7-[3-methyl-5-[2-methyl-5-[(pyridin-3-ylamino)methyl]phenyl]imidazol-4-yl]-4~{H}-1,4-benzoxazin-3-one 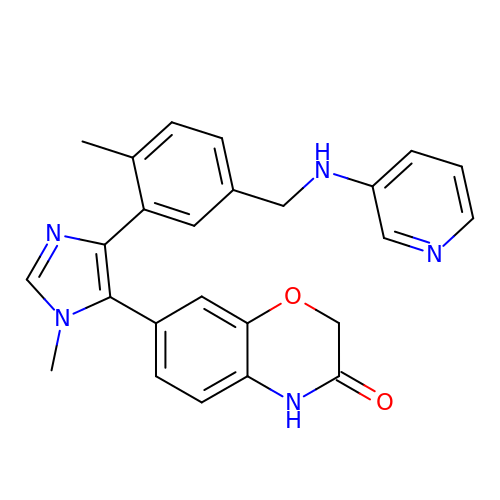| C25 H23 N5 O2 | APUAYMXUHLOPLQ-UHFFFAOYSA-N> HMRKIIVGSRRSKLALTQTKWVIEQLKKQGLPFEFEIKEMVTKGDQILNVTLSKVGGKGLFVKEIEQAMLDKEIDMAVHSMKEMPAVLPEGLTIGCIPLREDHRDALISKNGERFEELP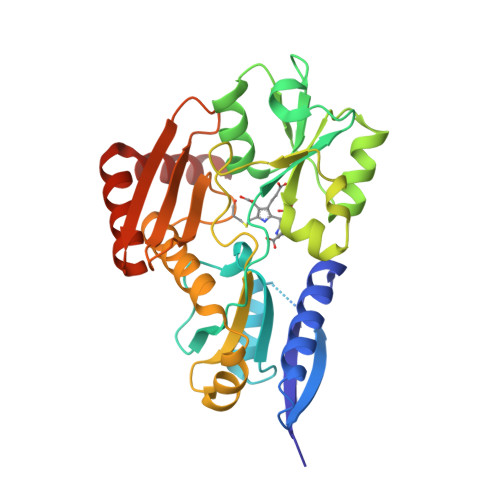SGAVIGTSSLRRGAQLLSMRSDIEIKWIRGNIDTRLEKLKNEDYDAIILAAAGLSRMGWSKDTVTQYLEPEISVPAVGQGALAIECRENDHELLSLLQALNHDETARAVRAERVFLKEMEGGCQVPIAGYGRILDGGNIELTSLVASPDGKTIYKEHITGKDPIAIGSEAAERLTSQGAKLLIDRVKEELDK> SGAIYVGNFRVVNRHLATHNDWANLVWEDSSRDLLVSSTTAQGCDTIARCNCQTGVYYCNSRRKHYPVSFSKPSLIYVEASEYYPARYQSHLMLAQGHSEPGDAGGILRCQHGVVGIVSTGGNG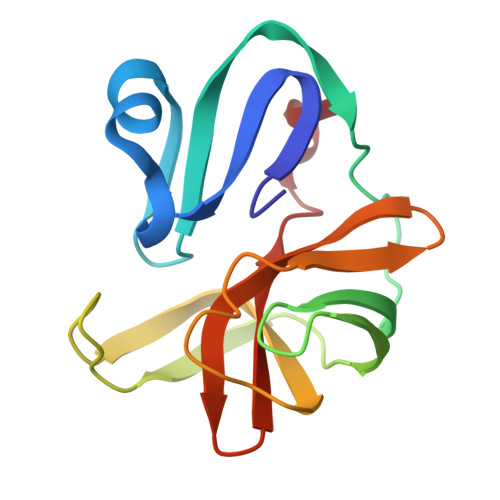LVGFADVRDLLWLD> MVSLPRMVYPQPKVLTPCRKDVLVVTPWLAPIVWEGTFNIDILNEQFRLQNTTIGLTVFAIKKYVAFLKLFLETAEKHFMVGHRVHYYVFTDQPAAVPRVTLGTGRQLSVLEVGAYKRWQDVSMRRMEMISDFCERRFLSEVDYLVAVDVDMEFRDHVGVEILT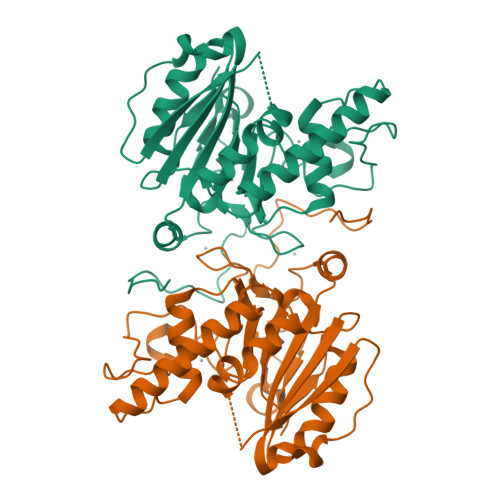PLFGTLHPSFYGSSREAFTYERRPQSQAYIPKDEGDFYYMGAFFGGSVQEVQRLTRACHQAMMVDQANGIEAVWHDESHLNKYLLRHKPTKVLSPEYLWDQQLLGWPAVLRKLRFTAVPKNHQAVRNP> ELTPDQQTLLHFIMDSYNKQRMPQEITNKILKEEFSAEENFLILTEMATNHVQVLVEFTKKLPGFQTLDHEDQIALLKGSAVEAMFLRSAEIFNKKLPSGHSDLLEERIRNSGISDEYITPMFSFYKSIGELKMTQEEYALLTAIVILSPDRQYIKDREAVEKLQEPLLDVLQKLCKIHQPENPQHFAELLGRLTELRTFNH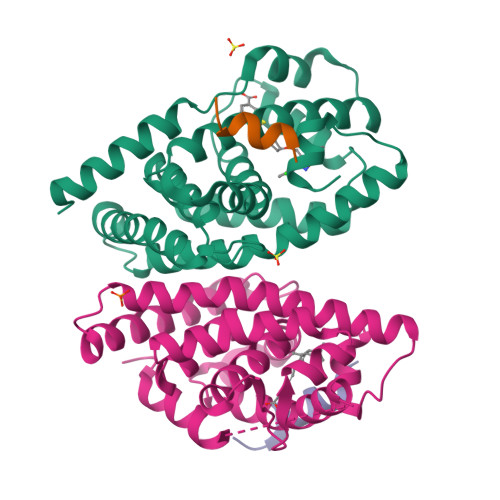HHAEMLMSWRVNDHKFTPLLEEIWDV;>[2x]ERHKILHRLLQEGSPS;> SANEDMPVERILEAELAVEPKTETYVEANMGLNPSSPNDPVTNICQAADKQLFTLVEWAKRIPHFSELPLDDQVILLRAGWNELLIASFSHRSIAVKDGILLATGLHVHRNSAHSAGVGAIFDRVLTELVSKMRDMQMDKTELGCLRAIVLFNPDSKGLSNPAEVEALREKVYASLEAYCKHKYPEQPGRFAKLLLRLPALRSIGLKCLEHLFFFKLIGDTPIDTFLMEMLEAPHQMT>SPSSSEGGAFTVNMPKTSTVDDIRGCPTLETPLKLTFTEDIQPRKENGSTYFYYDGWRGVGQTVNPWSPVLDNHKYAATEHEIHIYVEFFQTPSNRFADKNGAYSYIDANGVMYTNGEYSWEHVPALGKNIYKVVISDWNKGQTKSIYLPGRDFKTVEVFHFQNNRPQWDDRNSYENVKSRINNNISKSYSKAKLNEQLSTYVHDDGTDSLFLYQKLSRASLKESQINYYQLRGKFNGVNLGYWAQEYIL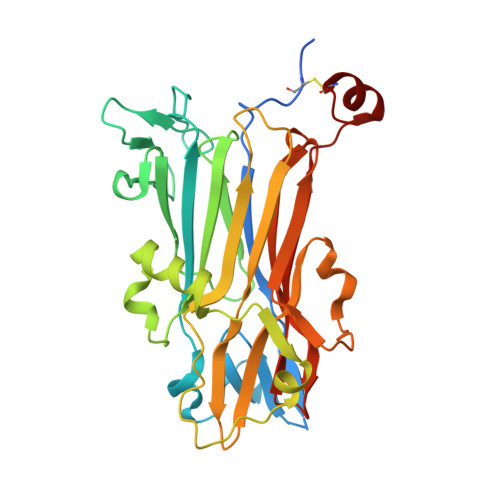FGGEGAEQLKNKIPDMSNYSMEDNGSFKNALKIESLDLRLMDNNRMAYGSTGTYIASFNRTDFSMTPENLKACGLD[8x]2-({[2-({(3S,4S)-4-[(6-amino-4-methylpyridin-2-yl)methyl]pyrrolidin-3-yl}oxy)ethyl]amino}methyl)phenol 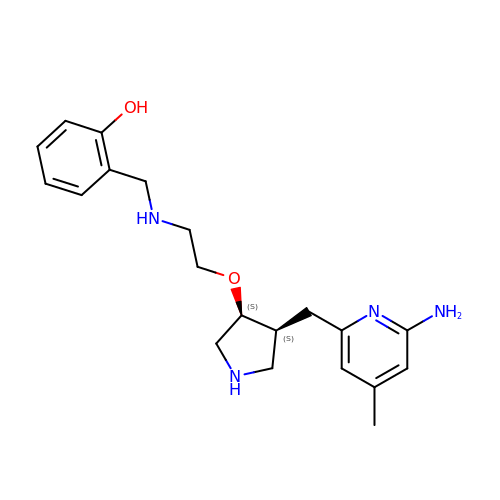| C20 H28 N4 O2 | YLQFJYDIDCSGLP-QFBILLFUSA-N> MLVAYDSMTGNVKRFIHKLNMPAVQIGEDLVIDEDFILITYTTGFGNVPERVLEFLERNNEKLKGVSASGNR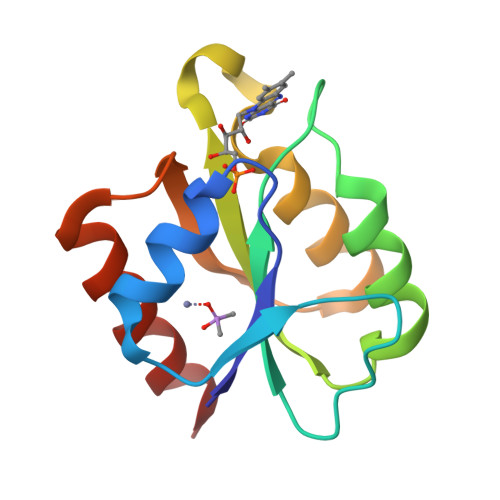NWGDMFGASADKISAKYEVPIVSKFELSGTNNDVEYFKERVREIATH>[3x]MKKILDSAKNYLNTHDKLKTACLIALELPSSSGSAATYIYLTDYFRDVTYNGILYRSGKVKSISSHKQNRQLSIGSLSFTITGTAEDEVLKLVQNGVSFLDRGITIHQAIINEEGNILPVDPDTDGPLLFFRGRITGGGIKDNVNTSGIGTSVITWNCSNQFYDFDRVNGRYTDDASHRGLEVVNGTLQPSNGAKRPEYQEDYGFFHSNKSTTILAKYQVKEERYKLQSKKKLFGLSRSYSLKKYYETVTKEVDLDFNLAAKFIPVVYGVQKIPGIPIFADTELNNPNIVYVVYAFAEGEIDGFLDFYIGDSPMICFDETDSDTRTCFGRKKIVGDTMHRLAAGTSTSQPSVHGQEYKYNDGNGDIRIWTFHGKPDQTAAQVLVDIAKKKGFYLQNQNGNGPEYWDSRYKLLDTAYAIVRFTINENRTEIPEISAEVQGKKVKVYNSDGTIKADKTSLNGIWQLMDYLTSDRYGADITLDQFPLQKVISEAKILDIIDESYQTSWQPYWRYVGWNDPLSENRQIVQLNTILDTSESVFKNVQGILESFGGAINNLSGEYRITVEKYSTNPLRINFLDTYGDLDLSDTTGRNKFNSVQASLVDPALSWKTNSITFYNSKFKEQDKGLDKKLQLSFANITNYYTARSYADRELKKSRYSRTLSFSVPYKFIGIEPNDPIAFTYERYGWKDKFFLVDEVENTRDGKINLVLQEYGEDVFINSEQVDNSGNDIPDISNNVLPPRDFKYTPTPGGVVGAIGKNGELSWLPSLTNNVVYYSIAHSGHVNPYIVQQLENNPNERMIQEIIGEPAGLAIFELRAVDINGRRSSPVTLSVDLNSAKNLSVVSNFRVVNTASGDVTEFVGPDVKLAWDKIPEEEIIPEIYYTLEIYDSQDRMLRSVRIEDVYTYDYLLTYNKADFALLNSGALGINRKLRFRIRAEGENGEQSVGWATI;>MTDKLIRELLIDVKQKGATRTAKSIENVSDALENAAAASELTNEQLGKMPRTLYSIERAADRAAKSLTKMQASRGMAGITKSIDGIGDKLDYLAIQLIEVTDKLEIGFDGVSRSVKAMGNDVAAATEKVQDRLYDTNRALGGTSKGFNDTAGAAGRASRALGNTSGSARGATRDFAAMAKIGGRLPIMYAALASNVFVLQTAFESLKVGDQLNRLEQFGTIVGTMTGTPVQTLALSLQNATNGAISFEEAMRQASSASAYGFDSEQLEQFGLVARRAAAVLGVDMTDALNRVIKGVSKQEIELLDELGVTIRLNDAYENYVKQLNATSTGIKYTVDSLTTYQKQQAYANEVIAESTRRFGYLDDALKATSWEQFAANANSALRSLQQSAATYLNPVMDTLNTFLYQTKSSQMRVSAMARSASAKTTPAENVTALIENAVGAREDLDTYLKESEERVKKAQELKQQLDDLKAKQAATAPIANALTAGGIGGDESNKLVVQLTNELARQNKEIEERTKTEKVLRQAVQDTGEALLRNGKLAEQLGAKMKYADTAVPGDKGVFEVDPNNLKAVSEIQKNFDFLKKSSSDTANNIRMAASSITNAKKASSDLNSVVKAVEDTSKVTGQSADTLVKNLNLGFSSLDQMKAAQKGLSEYVTAMDKSEQNALEVAKRKDEVYNQTKDKAKAEAAAREVLLRQQQEQLTAAKALLAINPNDPEALKQVAKIETEILNTKAQGFENAKKTKDYTDKILGVDREIALLNDRTMTSTQYRLAQLRLELQLEQEKTELYSKQADGQAKVEQSRRAQAQISREIWEAEKQGTASHVSALMDALEVSQTQRNVTGQSQILTERLSILQQQLELSKGNTEEELKYRNEIYKTSAALEQLKKQRESQMQQQVGSSVGATYTPTTGLIGEDKDFADMQNRMASYDQAISKLSELNSEATAVAQSMGNLTNAMIQFSQGSLDTTSMIASGMQTVASMIQYSTSQQVSAIDQAIAAEQKRDGKSEASKAKLKKLEAEKLKIQQDAAKKQIIIQTAVAVMQAATAVPYPFSIPLMVAAGLAGALALAQASSASGMSSIADSGADTTQYLTLGERQKNVDVSMQASSGELSYLRGDKGIGNANSFVPRAEGGMMYPGVSYQMGEHGTEVVTPMVPMKATPNDQLSDGSKTTSGRPIILNISTMDAASFRDFASNNSTAFRDAVELALNENGTTLKSLGNS[3x]

In siphophage T5, the unique RBP is located at the extremity of a central fiber. FhuA, an outer membrane E. coli iron-ferrichrome transporter, is the bacterial receptor recognized by T5 (25). We present the structures of T5 tail tip, determined by cryo–electron microscopy before and after interaction with its E. coli receptor, FhuA, reconstituted into nanodisc. These structures bring out the important conformational changes undergone by T5 tail tip upon infection, which include bending of T5 central fiber on the side of the tail tip, tail anchoring to the membrane, tail tube opening, and formation of a transmembrane channel.

The structures of the tip before and after interaction with FhuA start to diverge from BHPpb3 distal domains. More precisely, hdI and hIV overlay remarkably, with an RMSD of 0.85 Å over 244 residues. However, hdII and hdIII rotate around the long helix of hdIII as a rigid body (the RMSD before and after opening of hdII-III is 0.75 Å over 367 residues), and the plug unwinds in a long β-hairpin. These conformational changes result in BHPpb3 trimer opening, creating a channel with a constant ~40 Å in diameter from the hdI-hdIV ring to the hdII insertion tip. The three β-hairpin legs connect BHPpb3 to the nanodisc: Their tip is composed of 233-Leu-Phe-Gly-Leu-236, which would insert into the outer leaflet of the lipid bilayer hydrophobic core. In the crevice opened at the interface between two BHPpb3 subunits, extra densities were identified, in which the 43 C-terminal residues of TMPpb2* could be modeled. These densities merge with the ill-defined densities of BHPpb3 β-hairpin, strongly suggesting that TMPpb2* continues toward the nanodisc along BHPpb3 β-hairpin, forming with the latter a three-stranded β sheet. TMPpb2* is in turn expelled from the tail tube and anchor its C terminus in the crevice created between BHPpb3 monomers upon opening. Its hydrophobic segments would then insert in the outer membrane to form a transmembrane channel. Thus, T5 tail tube is anchored to the outer membrane by both BHPpb3 and TMPpb2*, in addition to FhuA-RBPpb5: It ensures that the tail tube is locked in register with the channel formed by TMPpb2* in the outer membrane.> VFGYVTEDGDTALHLAVIHQHEPFLDFLLGFSAGHEYLDLQNDLGQTALHLAAILGEASTVEKLYAA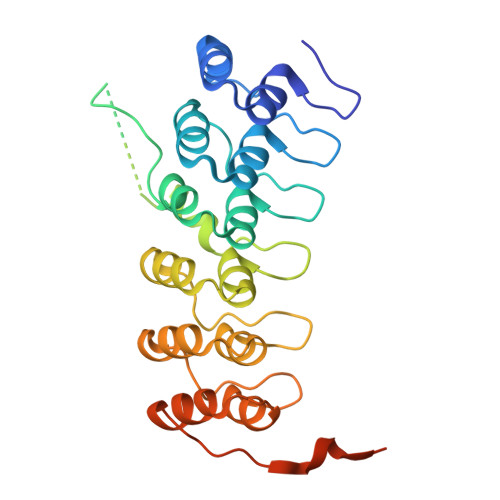GAGVLVAERGGHTALHLACRVRAHTCACVLLQPRPSHPRDASDTYLTQSQDCTPDTSHAPAAVDSQPNPENEEEPRDEDWRLQLEAENYDGHTPLHVAVIHKDAEMVRLLRDAGADLNKPEPTCGRTPLHLAVEAQAASVLELLLKAGADPTARMYGGRTPLGSALLRPNPILARLLRAHGAPEPEDGGDKLSPCEEEGEDEDSDNRDEGDEYDD>[4x]SYSTLANFPVQARNDNI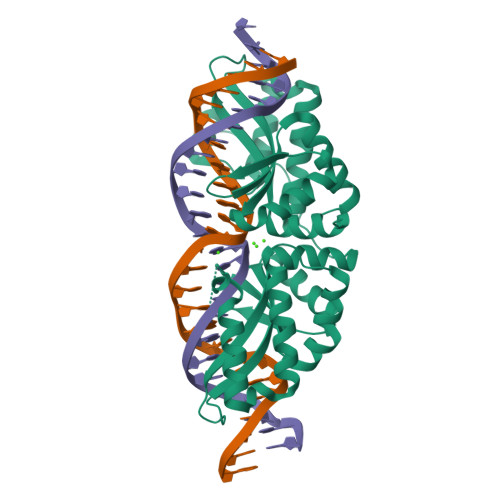SPWTITGFADAESSFMLTVSKDSKRNTGWSVRPRFRIGLHNKDVTILKSIREYLGAGIITSDIDARIRFESLKELEVVINHFDKYPLITQKRADYLLFKKAFYLIKNKEHLTEEGLNQILTLKASLNLGLSEELKEAFPNTIPAERLLVTGQEIPDSNWVAGFTAGDGSFYIRIAKNSTLKTGYQVQSVFQITQDTRDIELMKNLISYLNCGNIRIRKYKGSEGIHDTCVDLVVTNLNDIKEKIIPFFNKNHIIGVKLQDYRDWCKVVTLIDNKEHLTSEGLEKIQKIKEGMNRGRSL> AMALTGCSEKININEDKISHKIDIPDSAWTIGIGEKFKNAGHPNVKYPMIDDSYVQGAPLGGFGAGTIGRTYNGGFSRWHLEIGKNKYTTVYANQFSVFQKVEGNKDGVAQVLYAGEPENGYLSSWKWDYPKESGMYYALYPNSWYTYTNKDLPVQLAVKQFSPIIPYNYKETSYPVAVFKWTAYNPTNKNVDVSIMFTWQNMIGFFGKQVNVNSGNFNKIIKDKSKDSEIVAAVMGNISNDNEEWNGEYSIGVKKVPGVDISYKAKFVTTGDGSDLWHEFSKNGILDNKDDETPTKQDGIGSAIAVNFKLQPGQTIEVPFALSWDLPIMKFGGGDKWYKMYTKYFGKNGKNSFAILKEALNNYQKWEKMIDDWQKPILSNKSKPDWYKTALFNELYYLADGGTAWENGKVGEKDKRTNNMFGLLGCFDYNYYETLDVRFYGSFPLVMLWPDIEKQVMRQFADTINVQDSSEFKVGSNGAMAVKKVQGMIPHDLGSSYALPWIKINAYDWQNPNIWKDLNSKYVLLVYRDYVLTGKTDKEFLKYTWKSVKTALDKLKEMDKDNDGIPDNEGIPDQTYDTWSMKGTSAYCGSLWLAALKAAQEIGKVLKDNEAYIKYNEWYKIAQQNFEKELWNGEYYNFDTESDHKDSIMADQLAGQWYADILRLGDILPKDHVQKALKKIYEFNVMKFENGKMGAVNGMRPDGIVDESDIQA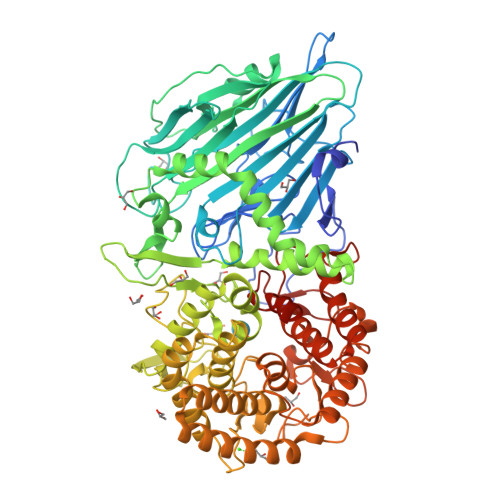QEVWTGVTYALASFMKYRGMTEEAYNTAYGVYKMTYDKSGKGYWFRTPEAWTKDGNYRASMYMRPLSIWSMEVNYNEVLEHHHHHH>[4x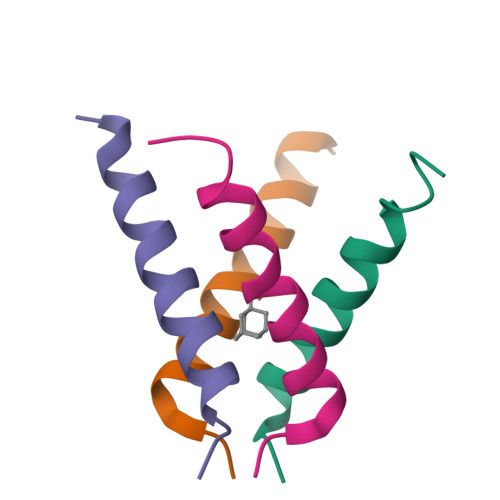]SSDPLVVAASIIAILHLILWILDRL E. coli aspartate aminotransferase (AAT) is a pyridoxal phosphate (PLP)-dependent enzyme that catalyses the reversible transamination of l-aspartate with α-ketoglutarate, yielding oxaloacetate and l-glutamate. During its catalytic cycle, AAT undergoes hinge movement to switch between an open conformation, in the ligand-free form, and a closed conformation upon association with substrates or inhibitors. Using our approach, we enrich the less populated but catalytically active closed conformation in order to increase catalytic efficiency (kcat/KM) with the non-native substrate l-phenylalanine, leading to altered substrate selectivity. Steady-state kinetics reveal kcat/KM increases of up to 100-fold towards this aromatic amino acid, resulting in a selectivity switch of up to 1900-fold, and structural analyses by room-temperature X-ray crystallography and multitemperature nuclear magnetic resonance (NMR) spectroscopy confirm that the conformational landscape is remodeled to favor the target state.

We collected X-ray diffraction data at room temperature (278 K) for all variants with the exception of AIFS, which could only be measured at cryogenic temperature (100 K) because we could only obtain small crystals that were not robust to radiation damage at non-cryogenic temperatures. To obtain structures in the absence of maleate, we applied a rigorous crystal soaking method to serially dilute and extract the inhibitor from the crystallized enzymes. Superposition of bound and unbound structures for each variant confirmed that closed library mutants VFIT and VFIY remained in the closed conformation in the inhibitor-free form, similar to HEX, while OpenLow variant VFCS and OpenHigh variant AIFS adopted the open conformation, similar to WT. AIFS is unique in that the electron density is especially weak in the regions corresponding to the helix formed by Pro12–Leu19 and the loop connecting moving and fixed domains (Leu31–Thr43), even at cryogenic temperatures, demonstrating that these structural segments are disordered when the enzyme adopts the open conformation. This result suggests that the four mutations of AIFS, three of which are found within the Leu31–Thr43 loop, contribute to destabilize the open conformation, consistent with the calculated Eopen value of this variant being >7 kcal mol–1 higher than that of the other variants that favor the open state (WT and VFCS). However, OpenHigh mutant AIFS gave rise to spectra that were distinct from those of all other variants, but could be deconvoluted to two exchanging peaks, to allow estimation of populations. We postulate that those peaks correspond to alternate open conformations distinct from the one sampled by the other variants.

>[2x]MAHHHHHHVGTFENITAAPADPILGLADLFRADERPGKINLGIGAYIDETGKFPVLTSVKKAEQYLLENETTKSYLGIDGIPEFGRCTQELLFGKGSALINDKRARTAQTPGGTGALRVAADFLAKNTSVKRVWVSNPSWPNHKSVFNSAGLEVREYAYYDAENHTLDFDALINSLNEAQAGDVVLFHGCCHNPTGIDPTLEQWQTLAQLSVEKGWLPLFDFAYQGFARGLEEDAEGLRAFAAMHKELIVASSYSKNFGLYNERVGACTLVAADSETVDRAFSQMKAAIRANYSNPPAHGASVVATILSNDALRAIWEQELTDMRQRIQRMRQLFVNTLQEKGANRDFSFIIKQNGMFSFSGLTKEQVLRLREEFGVYAVASGRVNVAGMTPDNMAPLCEAIVAVL N-[(naphthalen-2-ylamino)(oxo)acetyl]-beta-D-glucopyranosylamine | C18 H20 N2 O7 | 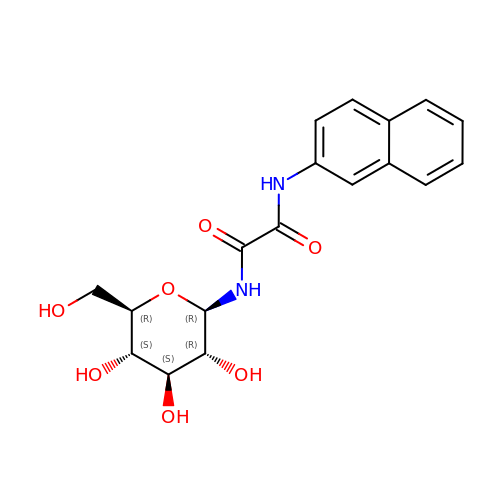WDRIXCWRSIXUDT-VPKNTQAGSA-N>[4x]NNLISFTMKRIVL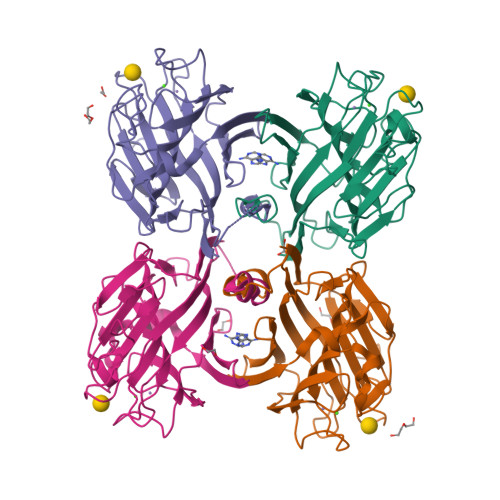FLILLTKAASANLISFTFKKFNETNLILQRDATVSSGKLRITKAAENGVPTAGSLGRAFYSTPIQIWDNTTGTVASWATSFTFNLQAPNAASPADGLAFALVPVGSQPKDKGGFLGLFDSKNYASSNQTVAVEFDTFYNGGWDPTERHIGIDVNSIKSIKTTSWDFANGENAEVLITYDSSTNLLVASLVHPSQKTSFIVSERVDLTSVLPEWVSVGFSATTGLSKGYVETNEVLSWSFASKLSINKEDEENKLAIFNLEGKAINNLA> SLSCDRNGICKGSSGSLNSIPSGLTEAVKSLDLSNNRITYISNSDLQRCVNLQALVLTSNGINTIEEDSFSSLGSLEHLDLSYNYLSNLSSSWFKPLSSLTFLNLLGNPYKTLGETSLFSHLTKLQILRVGNMDTFTKIQRKDFAGLTFLEELEIDASDLQSYEPKSLKSIQNVSHLILHMKQHILLLEIFVDVTSSVECLELRDTDLDTFHFSELSTGETNSLIKKFTFRNVKITDESLFQVMKLLNQISGLLELEFDDCTLNGVGNFRASDNDRVIDPGKVETLTIRRLHIPRFYLFYDLSTLYSLTERVKRITVENSKVFLVPCLLSQHLKSLEYLDLSENLMVEEYLKNSACEDAWPSLQTLILRQNHLASLEKTGETLLTLKNLTNIDISKNSFHSMPETCQWPEKMKYLNLSSTRIHSVTGCIPKTLEILDVSNNNLNLFSLNLPQLKELYISRNKLMTLPDASLLPMLLVLKISRNQLKSVPDGIFDRLTSLQKIWLHTNPW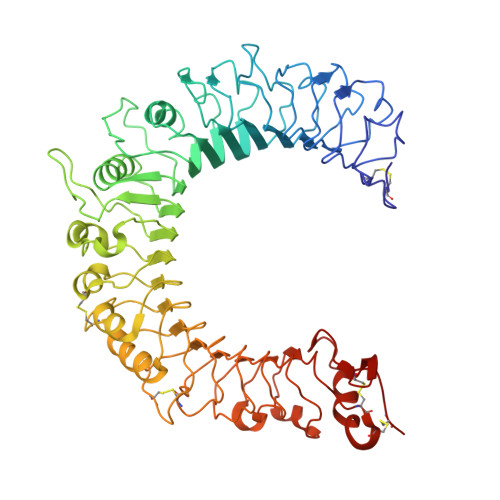DCSCPRIDYLSRWLNKNSQKEQGSAKCSGSGKPVRSIICP6-[(2-hydroxybenzyl)amino]pyridine-3-carboxamide | C13 H13 N3 O2 | 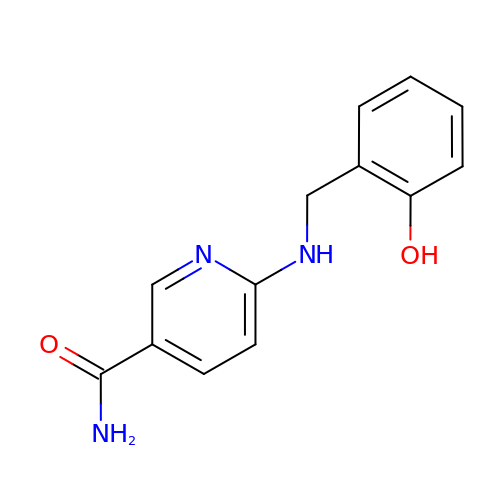NNNVBOGULIXEBW-UHFFFAOYSA-N>GSPSRAEYRNWSKPQCDITGFAPFSKDNSIRLSAGGDIWVTREPYVSCDPDKCYQFALGQGTTLNNVHSNNTVRGRTPYRTLLMNELGVPFHLGTKQVCIAWSSSSCHDGKAWLHVCITGDDKNATASFIYNGRLVDSVVSWSKEILRTQESECVCINGTCTVVMTDGSASGKADTKILFIEEGKIVHTSTLSGSAQHVEECSCYPRYPGVRCVCRDNWKGSNRPIVDINIKDHSIVSSYVCSGLVGDTPRKNDSSSSSHCLDPNNEEGGHGVKGWAFDDGNDVWMGRTINETSRLGYETFKVIEGWSNPKSKLQINRQVIVDRGNRSGYSGIFSVEGKSCINRCFYVELIRGRKEETEVLWTSNSIVVFCGTSGTY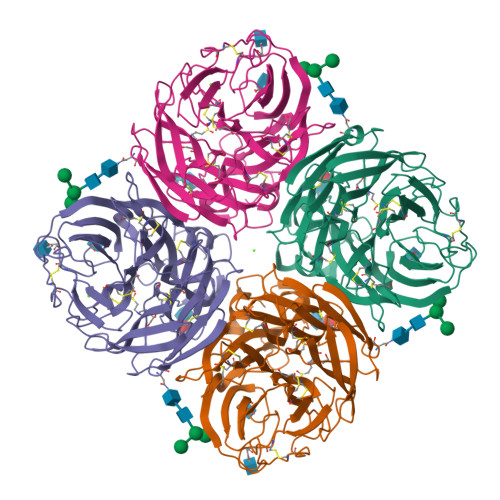GTGSWPDGADLNLMPI[4x]> GSHMASSDDVTVVYQNGLPVISVRLPSRRERCQFTLKPISDSVGVFLRQLQEEDRGIDRVAIYSPDGVRVAASTGMDLLLMDDFKLVINDLTYHVRPPKRDLLSHENAA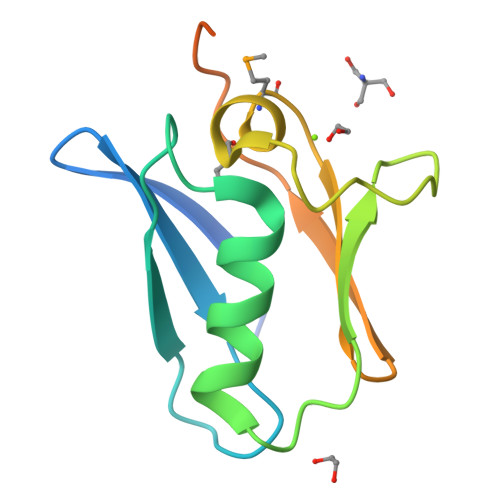TLNDVKTLVQQLYTT> GPAPANTQSGILNDGYFPPGTSKHELIARASSLKVSEVKAIIKKQVDEHWDVIRDVCGFKNKEVAYAFFFGMATRESTFRAATETGSGASHAFGPLQTAETAYANANPNYMP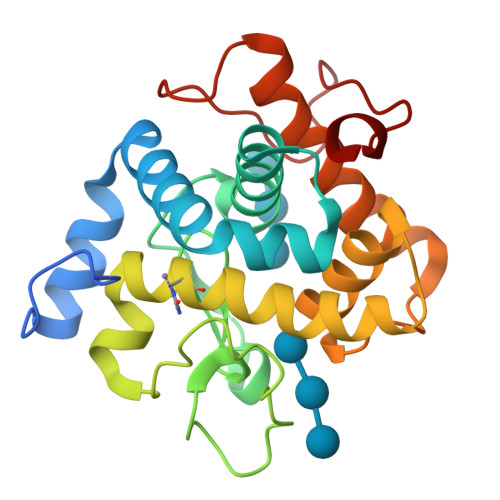EHNVPEMHQYDFTEYNFYDVGISVHMGIRHFLHFARLAKEKYSGRDIARHGLMGYNTGWIDGADESWIVRYADETAALGAWYLRNNHMSDDEFTWDTDPRVDRSNPWEIYY9,9'-(HEXANE-1,6-DIYLDIIMINO)BIS{N-[2-(DIMETHYLAMINO)ETHYL]ACRIDINE-4-CARBOXAMIDE} | C42 H50 N8 O2 | 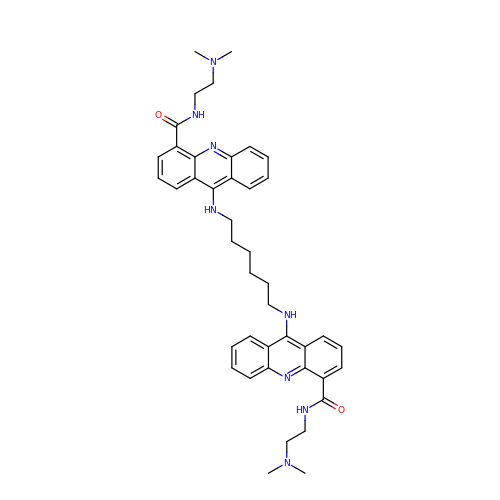ATHNVLFOCKEETH-UHFFFAOYSA-N>[16x]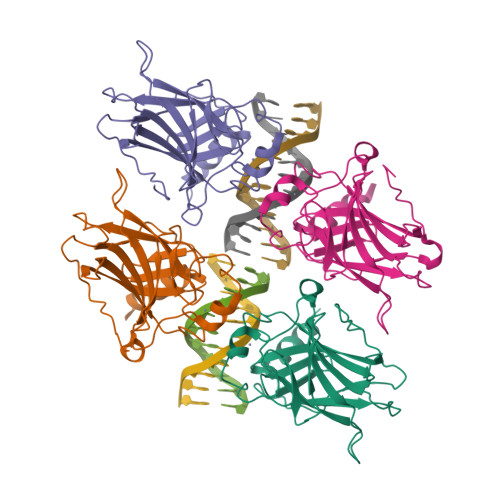MGHHHHHHHHEFIPSNTDYPGPHHFEVTFQQSSTAKSATWTYSPLLKKLYCQIAKTCPIQIKVSTPPPPGTAIRAMPVYKKAEHVTDVVKRCPNHELGRDFNEGQSAPASHLIRVEGNNLSQYVDDPVTGRQSVVVPYEPPQVGTEFTTILYNFMCNSSCVGGMNRRPILIIITLEMRDGQVLGRRSFEGRICACPGRDRKADEDHYREQ>MSTQYETQGYTINNAGRRLVVDPITRIQGHMRCEVNINDQNVITNAVSCGTMFRGLEIILQGRDPRDAWAFVERICGVCTGVHALASVYAIEDAIGIKVPDNANIIRNIMLATLWCHDHLVHFYQLAGMDWIDVLDALKADPRKTSELAQSLSSWPKSSPGYFFDVQNRLKKFVEGGQLGIFRNGYWGHPQYKLPPEANLMGFAHYLEALDFQREIVKIHAVFGGKNPHPNWIVGGMPCAINIDESGAVGAVNMERLNLVQSIITRTADFINNVMIPDALAIGQFNKPWSEIGTGLSDKCVLSYGAFPDIANDFGEKSLLMPGGAVINGDFNNVLPVDLVDPQQVQEFVDHAWYRYPNDQVGRHPFDGITDPWYNPGDVKGSDTNIQQLNEQERYSWIKAPRWRGNAMEVGPLARTLIAYHKGDAATVESVDRMMSALNLPLSGIQSTLGRILCRAHEAQWAAGKLQYFFDKLMTNLKNGNLATASTEKWEPATWPTECRGVGFTEAPRGALGHWAAIRDGKIDLYQCVVPTTWNASPRDPKGQIGAYEAALMNTKMAIPEQPLEILRTLHSFDPCLACSTH[2x];>LENKPRIPVVWIHGLECTCCTESFIRSAHPLAKDVILSLISLDYDDTLMAAAGTQAEEVFEDIITQYNGKYILAVEGNPPLGEQGMFCISSGRPFIEKLKRAAAGASAIIAWGTCASWGCVQAARPNPTQATPIDKVITDKPIIKVPGCPPIPDVMSAIITYMVTFDRLPDVDRMGRPLMFYGQRIHDKCYRRAHFDAGEFVQSWDD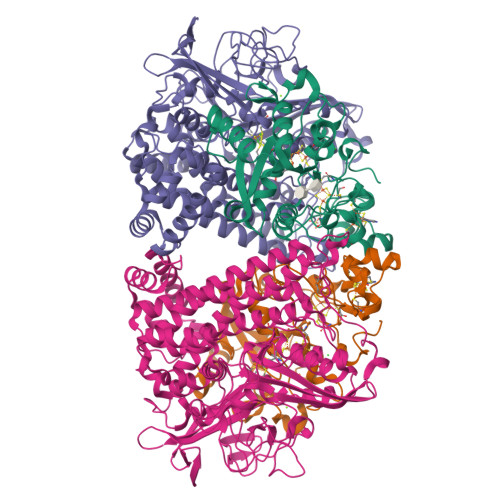DAARKGYCLYKMGCKGPTTYNACSSTRWNDGVSFPIQSGHGCLGCAENGFWDRGSFYSRVVDIPQMGTHSTADTVGLTALGVVAAAVGVHAVASAVDQRRRHNQQPTETEHQPGNEDKQARSHHHHHH[2x]Members of the family Birnaviridae possess bi-segmented double-stranded RNA (dsRNA) genomes and form virions with non-enveloped single-shelled icosahedral capsids. From sequence analysis it was proposed that the RdRPs of Birnaviridae possess a non-canonical active site where the polymerase sequence motifs are re-ordered C-A-B, motif C containing ADN in place of the conserved GDD catalytic residues. An additional unusual feature of birnavirus RdRPs is their ability to self-guanylylate: auto-catalyzing the covalent addition of a GMP moiety to a serine residue of the polymerase in a template-independent manner to form VP1pG. We have cloned, expressed and solved the structure of the RdRP VP1 from IPNV in both its apo form and bound to a catalytic metal (magnesium).

Crystals of full-length VP1 with the C-terminal hexahistidine tag removed diffracted to 3.8 Å resolution but proved refractory to further optimization. As for ΔC55 VP1 in the large unit cell, electron density for residues 3–19 was present in the active site. Some residual electron density could be observed linking residue 19 to the first residue (E27) of an adjacent polymerase molecule, but it was not sufficiently well-resolved to allow modeling of the intervening residues. Despite being crystallized in the presence of Mn2+ and ATP, no metal ions or nucleotides were observed at the active site. While additional electron density was seen connected to the C-terminus of the molecular replacement search model in three of the four copies of VP1 present in the asymmetric unit only eight additional residues (791–798) could be placed, suggesting that residues 799–845 are not ordered. Surprisingly the C-terminus of the fourth molecule in the asymmetric unit (from residue 687 onwards) is significantly refolded compared to the other IPNV VP1 molecules and IBDV VP1. The strand that runs along the side of the palm domain is shifted ‘upward’ to lie at the outer rim of the active site cleft. Neither the helix that lay between the base of the palm and fingers (residues 706–716), the three-helix bundle (residues 724–781) nor the intervening loop region are evident; instead the polypeptide has flipped up and projects away from the back of the fingers. Models of a VP1 elongation complex based on superposition of the reovirus RdRP elongation complex or of HIV reverse transcriptase in complex with a DNA template require refolding of a small segment of the VP1 C-terminal extension, residues 654–670, in order to accommodate the nascent RNA duplex (not shown). It is possible that the purpose of the C-terminal extension is to rigidify the polymerase during initiation, but that this extension must peel away to allow the growing nucleotide chain to exit the active site. The structure of VP1 where residues 688 onwards are refolded might thus represent an intermediate unfolding step rather than a conformation of biological significance in its own right.

>[3x]MSDIFNSPQNKASILTALMKSTTGDVEDVLIPKRFRPAKDPLDSPQAAAQFLKDNKYRILRPRAIPTMVELETDAALPRLRQMVEDGKLKDTVSVPEGTTAFYPKYYPFHKPDHDEVGTFGAPDITLLKQLTFFLLENDFPTGPETLRQVREAIATLQYGSGSYSGQLNRLLAMKGVATGRNPNKTPKTVGYTNEQLAKLLEQTLPINTPKHEDPDLRWAPSWLINYTGDLSTDKSYLPHVTIKSSAGLPYIGKTKGDTTAEALVLADSFIRDLGRAATSADPEAGVKKTITDFWYLSCGLLFPKGERYTQVDWDKKTRNIWSAPYPTHLLLSMVSTPVMNESKLNITNTQTPSLYGFSPFHGGMDRIMTIIRDSLDNDEDLVMIYADNIYILQDNTWYSIDLEKGEANCTPQHMQAMMYYLLTRGWTNEDGSPRYNPTWATFAMNVAPSMVVDSSCLLMNLQLKTYGQGSGNAFTFLNNHLMSTIVVAEWVKAGKPNPMTKEFMDLEEKTGINFKIERELKNLRETIVEAVETAPQDGYLADGSDLPPIRPGKAVELDLLGWSAIYSRQMEMFVPVLENERLIASAAYPKGLENKALARKPGAEIAYQIVRYEAIRLVGGWNNPLLETAAKHMSLDKRKRLEVKGIDVTGFLDDWNNMSEFGGDLEGITLSEPLTNQTLVDINTPLDSFDPKARPQTPRSPKKTLDEVTTAITSGTYKDPKSAVWRLLDQRTKLRVSTLRDQALALKPASSSVDNWAEATEELAQQQQLLMKANNLLKSSLTETREALETIQSDKIIAGKSNPEKNPGTAANPVVGYGEFSEKIPLTPTQKKNAKRREKQRRNQVEHHHHHH;> MSDIFNSPQNKASILTALMKSTTGDVEDVLIPKRFRPAKDPLDSPQAAAQFLKDNKYRILRPRAIPTMVELETDAALPRLRQMVEDGKLKDTVSVPEGTTAFYPKYYPFHKPDHDEVGTFGAPDITLLKQLTFFLLENDFPTGPETLRQVREAIATLQYGSGSYSGQLNRLLAMKGVATGRNPNKTPKTVGYTNEQLAKLLEQTLPINTPKHEDPDLRWAPSWLINYTGDLSTDKSYLPHVTIKSSAGLPYIGKTKGDTTAEALVLADSFIRDLGRAATSADPEAGVKKTITDFWYLSCGLLFPKGERYTQVDWDKKTRNIWSAPYPTHLLLSMVSTPVMNESKLNITNTQTPSLYGFSPFHGGMDRIMTIIRDSLDNDEDLVMIYADNIYILQDNTWYSIDLEKGEANCTPQHMQAMMYYLLTRGWTNEDGSPRYNPTWATFAMNVAPSMVVDSSCLLMNLQLKTYGQGSGNAFTFLNNHLMSTIVVAEWVKAGKPNPMTKEFMDLEEKTGINFKIERELKNLRETIVEAVETAPQDGYLADGSDLPPIRPGKAVELDLLGWSAIYSRQMEMFVPVLENERLIASAAYPKGLENKALARKPGAEIAYQIVRYEAIRLVGGWNNPLLETAAKHMSLDKRKRLEVKGIDVTGFLDDWNNMSEFGGDLEGITLSEPLTNQTLVDINTPLXXXXXXXXXXXXXXXXXXXXXXXXXXXXXXXXXXXXXXXXXXXXXXXXXXXXXXXXXXXXXXXXXXXXXXXXXXXXXXXXXXX> MHHHHHHHHHHGENLYFQGMKKITPKKEKYVIASDSTFAPFEFQNAQGDYVGIDVDLVKRAAELQGFTVEFKFIGFSSAVQAVESGQADGMVAGMTITDDRKKAFDFSVPYFDSGIQIAVKKGNDKIKSYDDLKGKKVGVKIGTES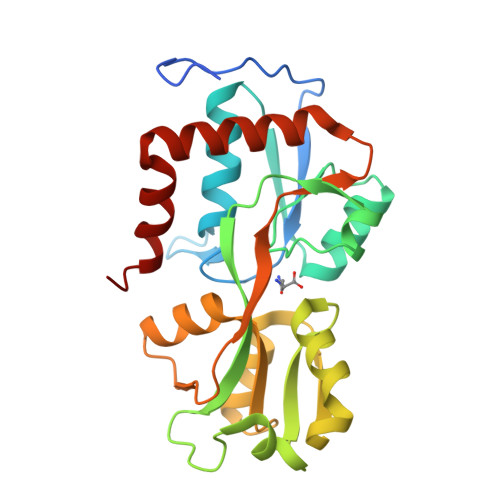ADFLEKNKKKYDYSIKYLDTTDALYSALEIGEVDAMMDDYPVIGYGVAQNQPLATPIPREKGGSYGFAVKKGQNPELLEMFNEGLKEMKRTGEYDKIIGTYVKDG> MGSSHHH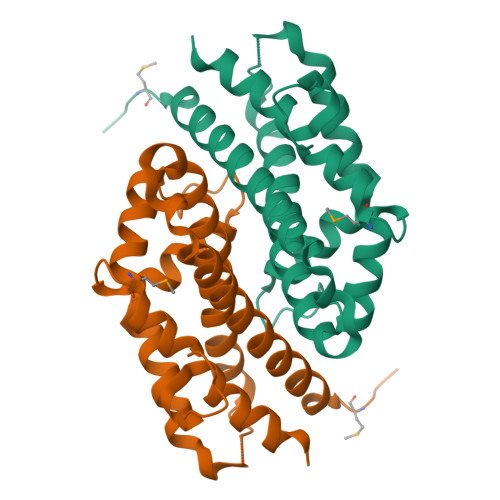HHHSSGRENLYFQGVKMSDKWIEIEEILSGLIGDLTIAVTVLKDYEGKAFLREPQHQTKRQCIWRLCVYSIVINCRKYVELNQKYGKEFQALIPGHNHIRGVYNNEINKNTAIKKLRNHCVAHVSDKSKYLKPAEVQEEIIKMFDGNFADEFLDWICPDNISTTDKSESLVGVIELLRDAVSAKL2,5-anhydro-1,3,4-trideoxy-2-(2,4-difluorophenyl)-6-O-{4-[4-(4-{1-[(1S,2S)-1-ethyl-2-hydroxypropyl]-5-oxo-1,5-dihydro-4H-1,2,4-triazol-4-yl}phenyl)piperazin-1-yl]phenyl}-1-(1H-1,2,4-triazol-1-yl)-D-erythro-hexitol 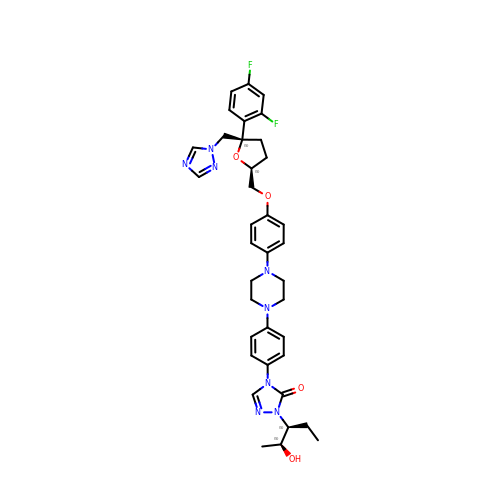| C37 H42 F2 N8 O4 | IEAWASLYDSYMSP-OLBKAPGZSA-N> PISPIETVPVKLKPGMDGPKVKQWPLTEEKIKALVEICTEMEKEGKISKIGPENPYSTPVFAIKKKDSTKWRKLVDFRELNKRTQDFWEVQLGIPHPAGLKKKKSVTVLDVGDAYFSVPLDEDFRKYTAFTIPSINNETPGIRYQYNVLPQGWKGSPAIFQSSMTKILEPFKKQNPDIVIYQYMDDLYVGSDLEIGQHRTKIEELRQHLLRWGLTTPDKKHQKEPPLLWMGYELHPDKWTVQPIVLPEKDSWTVNDIQKLVGKLNWASQIYPGIKVRQLCKLLRGTKALTEVIPLTEEAELELAENREILKEPVHGVYYDPSKDLIAEIQKQGQGQWTYQIYQEPFKNLKTGKYARMRGAHTNDVKQLTEAVQKITTESIVIWGKTPKFKLPIQKETWETWWTEYWQATWIPEWEFVNTPPLVKLWYQLEKEPIVGAETFYVDGAANRETKLGKAGYVTNKGRQKVVPLTNTTNQKTQLQAIYLALQDSGLEVNIVTDSQYALGIIQAQPDKSESELVNQIIEQLIKKEKVYLAWVPAHKGIGGNEQVDKLVSAGIRHHHHH;> PISPIETVPVKLKPGMDGPKVKQWPLTEEKIKALVEICTEMEKEGKISKIGPENPYNTPVFAIKKKDSTKWRKLVDFRELNKRTQDFWEVQLGIPHPAGLKKKKSVTVLDVGDAYFSVPLDEDFRKYTAFTIPSINNETPGIRYQYNVLPQGWKGSPAIFQSSMTKILEPFKKQNPDIVIYQYMDDL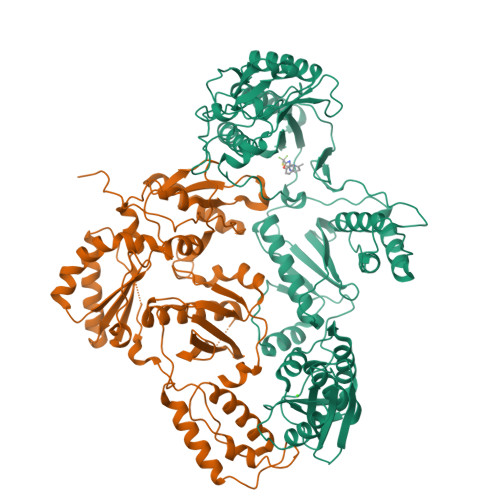YVGSDLEIGQHRTKIEELRQHLLRWGLTTPDKKHQKEPPFLWMGYELHPDKWTVQPIVLPEKDSWTVNDIQKLVGKLNWASQIYPGIKVRQLSKLLRGTKALTEVIPLTEEAELELAENREILKEPVHGVYYDPSKDLIAEIQKQGQGQWTYQIYQEPFKNLKTGKYARMRGAHTNDVKQLTEAVQKITTESIVIWGKTPKFKLPIQKETWETWWTEYWQATWIPEWEFVNTPPLVKLWYQ>[2x]GVQPLATQCFQLSNMFNPQTEEEVGWDTEIKDDVIEEC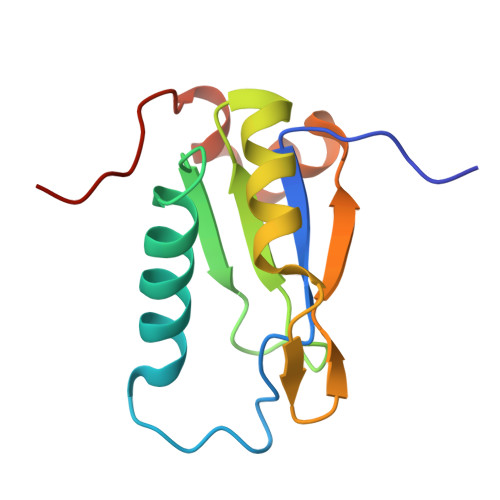NKHGGVIHIYVDKNSAQGNVYVKCPSIAAAIAAVNALHGRWFAGKMITAAYVPLPTYHNLFPDSMTATQLLVPSRR N-(2-{3-[(2-aminopyrimidin-5-yl)oxy]phenyl}ethyl)-3-(trifluoromethoxy)benzamide | C20 H17 F3 N4 O3 | 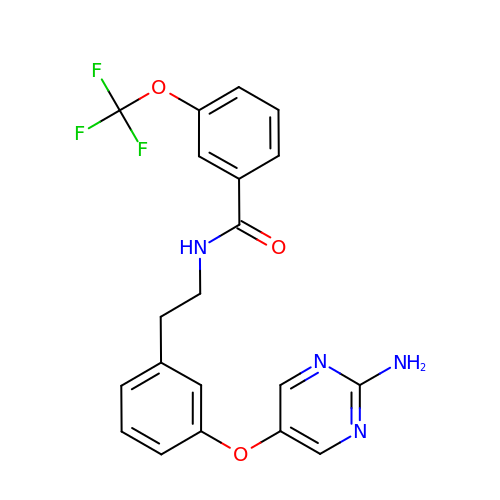JABJAPNNNDHTEK-UHFFFAOYSA-N Species D (HAdV-D) are the most diverse species and cause both gastrointestinal tract infections and epidemic keratoconjunctivitis (EKC). Each protein forms key interactions to promote cell infection, with the terminal domain of the fiber, the fiber knob protein, interacting with the viruses’ primary cell entry receptor. The adenovirus fiber knob protein is known to have a highly conserved trimeric structure. Sialic acid (SA) usage has been proposed as a major mechanism of cell infection for EKC causing HAdV-D. Here, we provide apo state crystal structures for fiber knob proteins of 7 previously undetermined HAdV-D, and provide crystal structures of HAdV-D25, HAdV-D29 and HAdV-D53 knob proteins bound to SA.

We performed X-ray crystallography to generate structures of species D human adenovirus fiber knob proteins HAdV-D15, D24, D29, D30, D32 and D53 in their apo states. These structures show the expected trimeric form, all viewed down towards the apical domain of the fiber knob proteins ([Fig fig1]). HAdV-D15, D24 and D32 were crystallised in only their apo states, whereas HAdV-D25, D29, D30 and D53 crystals were also soaked with sialic acid. Adenovirus fiber knob proteins crystallised readily, under widely varying pH conditions. The achieved resolution is mostly very high, up to 1.37-1.6Å, although some species gave diffraction to a more modest resolution. Pseudotyped viruses comprising an HAdV-C5 core viral vector psedutoyped with the fiber knob proteins of several HAdV-D of interest (D26, D15, D24, D29 and D53) were generated expressing a luciferase transgene under the control of a ubiquitous CMV IE promoter for measuring transduction following cell treatment with and without neuraminidase treatment. Non-significant changes in transduction were observed when cells were transduced with viruses with the fiber-knob proteins of HAdV-D15, D24 and D29 ([Fig fig3]). There was an overall trend in reduction, although in BT-20 cells there was a small, non-significant, increase in transduction of HAdV-D29 fiber-knob protein virus following treatment with neuraminidase. These results indicate significant usage of sialic acid by HAdV-D53 fiber-knob proteins, and the potential partial usage across the other species D adenovirus fiber-knob proteins.

>DKLTLWTTPDPSPNCKIIEDKDSKLTLILTKCGSQILGSVSLLVVKGKFSNINNTTNPNEADKQITVKLLFDANGVLKQGSTMDSSYWNYRSDNSNLSQPYKKAVGFMPSKTAYPKQTKPTNKEISQAKNKIVSNVYLGGKIDQPCVIIISFNEEADSDYSIVFYFKWYKTYENVQFDSSSFNFSYIAQE[3x]> MQDLEGKVAFVTGGGSGVALGQAKVLAEEAQMKVVIADIRQDHLDEAMGYFSQKNVAVHPVRLDLTDRAAYAAAVDEAEQVFGPVDLLCNTAGVSQFGPIEKATFDDWDWQMDVNVNGVINGVMTVMPRMIERGQGGHILITASMSAFVALPTTGIYCTTKYAVRGLAESLRVEMPKYNIGVSLLCPGGVNTNIHRSVEARPEKYGNTGYYGRDEAVFAGLKRVIEHGFDPVDLGRVVLDAVRNDRFWVLPYPEFAEGQKARDQEVIDAMMSYADHPDYARRMKIREQMKRDMPGSD

A cellular pathway has been characterized that performs β-aryl ether (β-ether)3 bond cleavage using three sequential Lig enzymes. The first step in the Lig pathway is a stereospecific oxidation of the benzylic alcohol in the GGE substrate to produce β-(2-methoxyphenoxy)-γ-hydroxypropiovanillone (MPHPV), which is catalyzed by nicotinamide adenine dinucleotide (NAD+)-dependent Cα-dehydrogenases LigD, LigL, LigN, and LigO. The final step consists of a GSH-dependent lyase, LigG, that catalyzes the elimination of the GSH thioether linkage in (βR)-GS-HPV to produce glutathione disulfide (GSSG) and γ-hydroxypropiovanillone (HPV). Our structural and biochemical studies of the enzymes in the bacterial β-aryl ether cleavage pathway reveal the features important for substrate and cofactor binding and catalysis by these Lig enzymes.

The LigD and LigO enzymes catalyze the oxidation of the (αR)-substrates (αR,βR)-GGE and (αR,βS)-GGE, whereas LigL and LigN are specific for the α(S)-configured substrates (αS,βR)-GGE and (αS,βS)-GGE. We have solved the crystal structures of LigD, LigO, and LigL, which by amino acid sequence alignment belong to the short chain dehydrogenase/reductase (SDR) superfamily of enzymes. The SDR family is characterized as a large group of NAD(P)H (2′-phosphorylated NADH)-dependent enzymes displaying an α/β folding pattern containing a Rossman fold; this overall organization is seen in the LigD, LigO, and LigL crystal structures. The superposition of the LigD, LigO, and LigL structures using Cα atoms shows a root mean square deviation for LigD-LigO of 0.88 Å, for LigD-LigL of 0.70 Å, and for LigO-LigL of 0.93 Å, indicating that the enzymes display similar overall structural features. A sequence alignment of LigD, LigO, and LigL shows an identity between LigD-LigO of 40%, LigD-LigL of 38%, and LigO-LigL of 37%. In these alignments, the most sequence-divergent region is in the predicted substrate binding loop. This proposed substrate binding region is disordered in all of the crystal structures solved in the apo-form (LigD, LigO, and LigL) and in the structures of the LigD·NADH and LigO·NADH complexes.>[2x]SNAMIFPKQYPIINFTTAGATVQSYTNFIRAVRGRLTTGADVRHEIPVLPNRVGLPINQRFILVELSNHAELSVTLALDVTNAYVVGYRAGNSAYFFHPDNQEDAEAITHLFTDVQNRYTFAFGGNYDRLEQLAGNLRENIE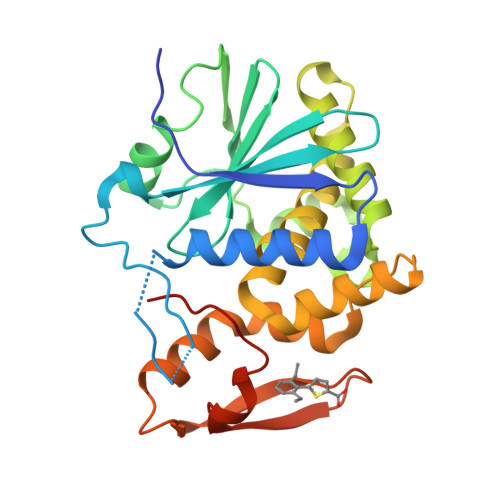LGNGPLEEAISALYYYSTGGTQLPTLARSFIICIQMISEAARFQYIEGEMRTRIRYNRRSAPDPSVITLENSWGRLSTAIQESNQGAFASPIQLQRRNGSKFSVYDVSILIPIIALMVYRCAPPPSSQF Phytochromes are red-light photoreceptors found in various plants and microorganisms. S. aurantiaca contains two previously uncharacterized bacteriophytochromes (BphPs) denoted SaBphP1 and SaBphP2, which may be responsible for the light-stimulated growth of multicellular fruiting bodies. The classical BphPs switch between a red absorbing state denoted Pr (λmax ≃ 700 nm) and a far-red absorbing state denoted Pfr (λmax ≃ 750 nm).

In order to understand the role of the unusual Thr289 in signal transduction in SaBphP1, we replaced it with a His so that the T289H variant SaBphP1 resembles classical BphPs. We denote these constructs as CBD-wt, CBD-T289H, PCM-wt and PCM-T289H. The wild-type and mutant CBDs both crystallize in the dark in the Pr state in space group P3221. When Thr289 is replaced by His, structural displacements throughout the chromophore binding pocket are observed. BV ring D moves almost 1 Å deeper into the pocket, and its carbonyl forms a hydrogen bond with His289 (∼2.8 Å) and with Ser287 (3.1 Å). In addition, the electron density of the water that hydrogen bonds to Ser287 near ring D is stronger in the mutant and there is an additional water molecule with respect to wild-type suggesting a more rigid and defined BV environment. However, the T289H mutation hardly changes the overall structure of the CBD dimer as the root-mean-square deviation (r.m.s.d.) between wild-type and mutant is on the order of 0.3 Å. Since the CBDs do not form stable Pfr spectra, but the PCMs do, the PHY domain is essential for the mechanics of the photoswitch.

> TNCDREPIHIPGAIQPHGVLLVLSEPGLVLTHASENAPAVLGNSAEQLLGAPLGHFIEPSVREPLEADLRSARLKQLNPLKVVWRVDGVDRFFDGIAHRHQGRLILELEPSSHREAVPFLSFFHAVRDGLSRLRDARDLQELCEAVVQEVRGLTGFDRAIIYRFDAEWNGSVIAEARDARADPYLGLHFPASDIPRQARELYQLNWLRIIPTIDYQPARVRALPGHGEPLDLSFSVLRSVSPIHLEYLHNMGVQASMSISLMKDGKLWGLISCHQVSGTRYVPYEVRTACEFLGEVMSSLLAA> GSHMASMSKDEVKREAKDTDGNPEIKGERRRLHSEI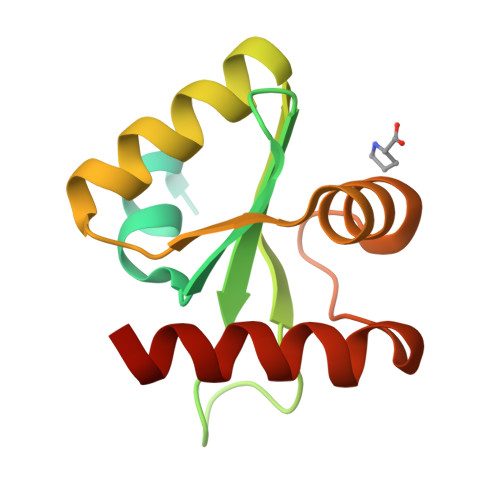QSGSLANNIKKSTVIVKNATHIAICLYYKLGETPLPLVIETGKDAKALQIIKLAELYDIPVIEDIPLARSLYKNIHKGQYITEDFFEPVAQLIRIAIDLDY;> GSHMASMSKDEVKREAKDTDGNPEIKGERRRLHSEIQSGSLANNIKKSTVIVKN;> ATHIAICLYYKLGETPLPLVIETGKDAKALQIIKLAELYDIPVIEDIPLARSLYKNIHKGQYITEDFFEPVAQLIRIAIDLDY> MPFVNKQFNYKDPVNGVDIAYIKIPNVGQMQPVKAFKIHNKIWVIPERDTFTNPEEGDLNPPPEAKQVPVSYYDSTYLSTDNEKDNYLKGVTKLFERIYSTDLGRMLLTSIVRGIPFWGGSTIDTELKVIDTNCINVIQPDGSYRSEEL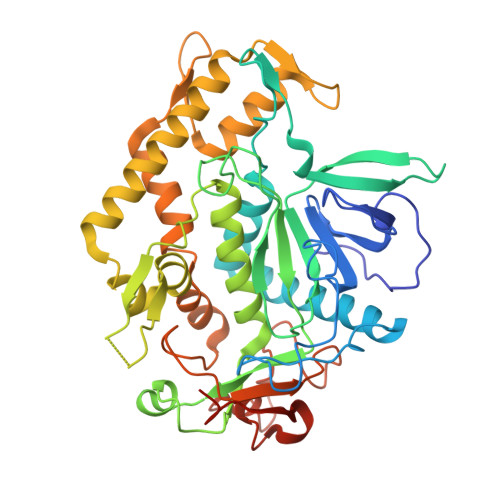NLVIIGPSADIIQFECKSFGHEVLNLTRNGYGSTQYIRFSPDFTFGFEESLEVDTNPLLGAGKFATDPAVTLAHELIHAGHRLYGIAINPNRVFKVNTNAYYEMSGLEVSFEELRTFGGHDAKFIDSLQENEFRLYYYNKFKDIASTLNKAKSIVGTTASLQYMKNVFKEKYLLSEDTSGKFSVDKLKFDKLYKMLTEIYTEDNFVKFFKVLNRKTYLNFDKAVFKINIVPKVNYTIYDGFNLRNTNLAANFNGQNTEINNMNFTKLKNFTGLFELEHHHHHH O-benzyl-N-methyl-L-tyrosinamide | C17 H20 N2 O2 | 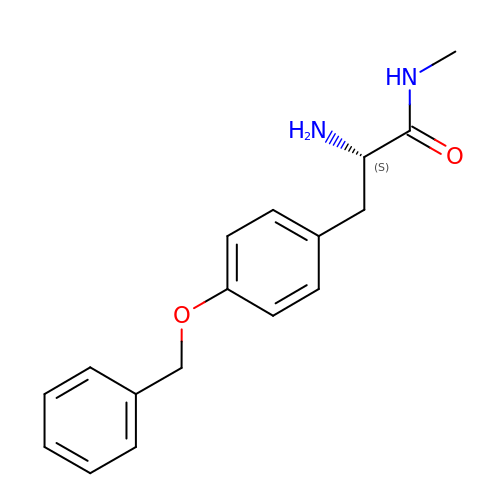ZMTWQALRHGTUHL-INIZCTEOSA-N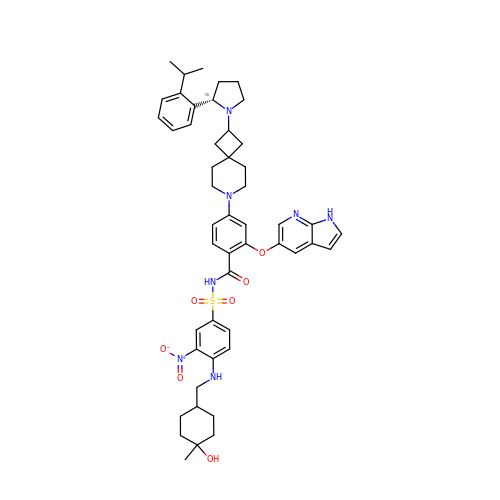~{N}-[4-[(4-methyl-4-oxidanyl-cyclohexyl)methylamino]-3-nitro-phenyl]sulfonyl-4-[2-[(2~{S})-2-(2-propan-2-ylphenyl)pyrrolidin-1-yl]-7-azaspiro[3.5]nonan-7-yl]-2-(1~{H}-pyrrolo[2,3-b]pyridin-5-yloxy)benzamide | C49 H59 N7 O7 S | ZQTKOYMWCCSKON-XKXNWSITSA-N> ENSHIENEDKRLTSEQKEIVHFVSEGVTPSTTALPDIVNLSTNYLDKNTREDRIHSIKDFLSRPIIIATNLWSVSDPVEKQLYTANFPEVLISNAMYQDKLKGFVGLRAT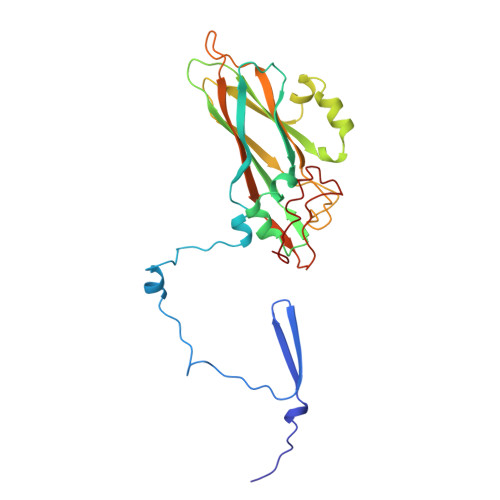LVVKVQVNSQPFQQGRLMLQYIPYAQYMPNRVTLINETLQGRSGCPRTDLELSVGTEVEMRIPYVSPHLYYNLITGQGSFGSIYVVVYSQLHDQVSGTGSIEYTVWAHLEDVDVQYPTGANIFTGNEAYIKGTSRYDAAQKAHAA>[4x]MDIKINDITLGNNSPFVLFGGINVLESLDSTLQTCAHYVEVTRKLGIPYIFKASFDKANRSSIHSYRG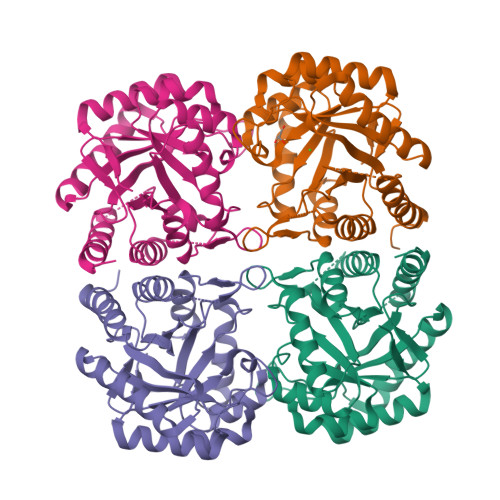VGLEEGLKIFEKVKAEFGIPVITDVHEPHQCQPVAEVCDVIQLPAFLARQTDLVVAMAKTGNVVNIKKPQFLSPSQMKNIVEKFHEAGNGKLILCERGSSFGYDNLVVDMLGFGVMKQTCGNLPVIFDVTHSLQTRDAGSAAAGGRRAQALDLALAGMATRLAGLFLESHPDPKLAKCDGPSALPLHLLEDFLIRIKALDDLIKSQPILTIE>[3x]MSGDTTLVDTVNASQSRQVFWDRDVYDLEIERIFSRAWLMLGHKSLLPKPGDFITTYMAEDKIILSHQSDGTFRAFINSCTHRGNQICHADSGNAKAFVCNYHGWVYGQDGSLVDVPLESRCYHNKLDKQELAAKSVRVETYKGFIFGCHDPEAPSLEDYLGEFRFYLDTIWEGGGAGLELLGPPMKSLLHCNWKVPVENFVGDGYHVG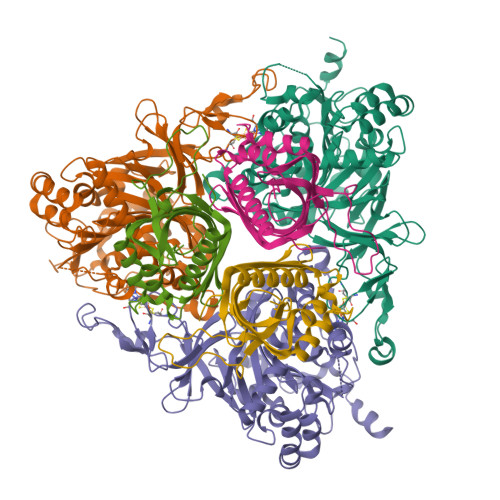WTHAAALGQIGGPLAGLAGNRADIPFDDLGLQFTTRHGHGFGVIDNAAAAIHRKGDGWNKYLEDTRGEVRRKFGADRERLYVGHWNGAIFPNCSFLYGTNTFKIWHPRGPHEIEVWTYTMVPSDADPATKSAIQREATRTFGTAGTLESDDGENMSSATYVNRGVITRDGMMNSTMGVGYEGPHPVYPGIVGISFIGETSYRGFYRFWKEMIDAPDWASVKANDDNWDSVFTNRNFWNEKLNAAE;>MSTEQVPVTPDVHYAVEAHYRAEVRLLQTGQYREWLHGMVAEDIHYWMPIYEQRFVRDRRPDPTPDDAAIYNDDFEELKQRVERLYSGQVWMEDPPSKIRYFVSNVEAFEAENGELDVLSNILVYRNRRQTEVTVHTLGREDKLRQDGNGFKVFRRKLILDARVTQDKNLYFFC[3x]>GSMTSKIALFDQTLIASLLQPLSLNQPDFKAYKTKVKLKISEQRNETSGEKELKFEISRSDDFEFLFSETLNNEKYQILARDHDLTVDFDAFPKVIIQHLLCKNIVKNLEEDGEVDARKKAGYHEIADPGKPTEINIILDAEKNFCSFELF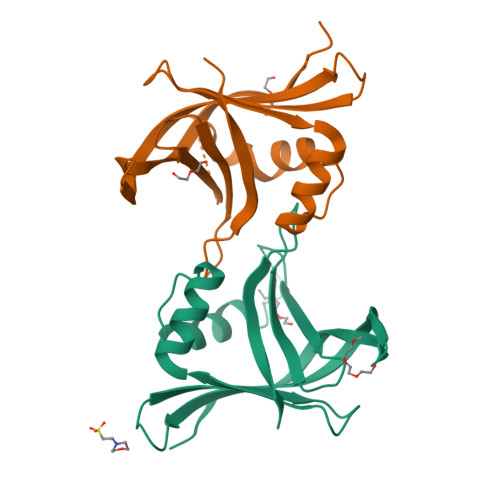SKTPISKGKIFSIKLHAVR[2x]> EDGDPAKGEAVFKKCMACHRVGPDAKNLVGPALTGVIDRQ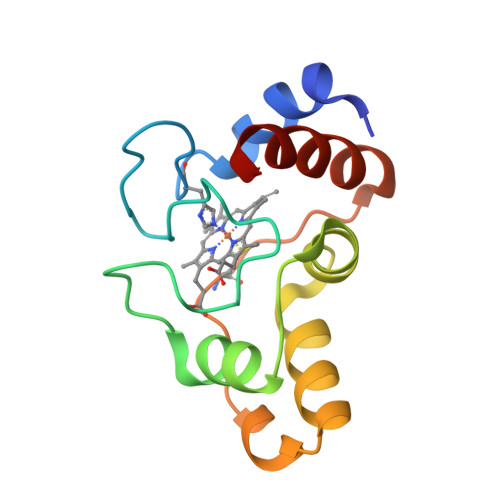AGTAPGFNYSAINHAAGEAGLHWTPENIIAYLPDPNAFLRKFLADAGHAEQAKGSTKMVFKLPDEQERKDVVAYLKQFSPQ> MANFLKNLHPLLRRDRNKKDNQDPNFALIDALNEEMNQVEKDAIESKLQSSLKTSTSEYLDKFGDWFGVYRKTDEKDDVYRARIIKYLLLKRGTNNAIIDAIKDYLGRDDIDVSVYEPFTNIFYTNKSHLNGEDHLMGYYYRFAVINVSIGDYFPVEIIDVINEFKPAGVTLYVTYDGASTIRGGAIIKWDDGLPKIETYQEFDRFTGYDDTFYGHINMNQSKDTDNSSSDIFKTNHSLINSLDVLTGSSSVGRQYINYGYVTSYVYNPGMTSSVNQISASTEGRGQEVPTDYYMYTSTKNNNTVELSMQTTSGVSYLYNNFNFRDYMSKYRPQVDLQSDEARRIVSDYIKELSIDYYLSAVIPPDESIEIKLQVYDFSINRWLTVSINNLSFYEKNIGSNIGYIKDYLNSELNMFTRLEINAGKRDSVDIKVNYLDLMFYYYERGIYTIKPYKALIENYLDISRETYVEAFKIASLSNGDIITKTGFQPIGYLKLVGNYENTIPSTINIVAKDTDNNPIESNELDVYNTVENRNLLQSYKGVNTIAREITSTKEFTVSGWAKEIYSTNYLSKVLKPGKVYTLSFDMEITGNDPTLKSYSDNHGIYLYSNTKGIVVNGVKSMERTIGNKVSVTQTFTAPTITDHRLLIYTGRYTSDGKASTPPVFFNTVKITELKLTEGSSKLEYSPAPEDKPNVIEKGIKFNNILTNIQTLSINSDTILKNVTLYYSYYGDSWVELKTLGNISTGETTETNNLIDLYGLQTVDYSNINPMSKVSLR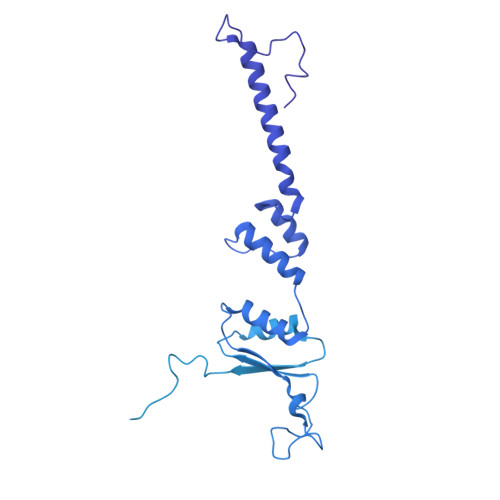SIWNVKLGELNNQEGSLSNMPNDYFNAVWQDIDKLSDIELGSMRMVKDTEGGVFDGATGEIIKATLFNVGAYTDLDMLAYTLTNYTEPLTLGSSRLISELKEELLTSESFNVDNRIKVIDSIYEELPNTSIIKNGFVEREVTGSKYLDYGLYEPIEDGTRYKLIVEGEFKDNIEFISLYNSNPNFNETFIYPSEIINGVAEKEFIAKPSTEDKPRLNTDVRIYIRPYDSTISKVRRVELRKV> MAEKFDHLEEHLEKFVENIRQLGIIVSDFQPSSQAGLSQKLNFIVTGLQDIDKCRQQLHDITVPLEVFEYIDQGRNPQLYTKECLERALAKNEQVKGKIDTMKKFKSLLIQELSKVFPEDMAKYRSIRGEDHPP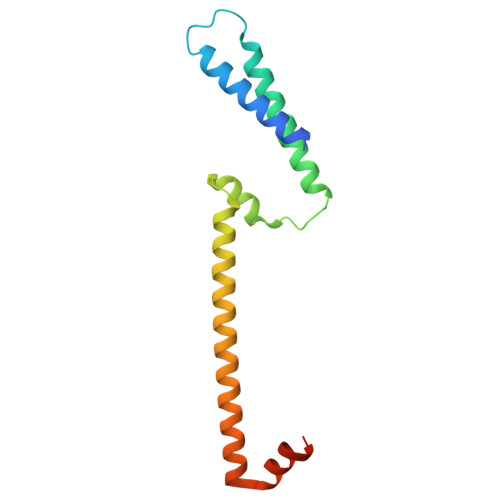S>[2x]MKTSKTKTPKSVLIAGPCVIESLENLRSIATKLQPLANNERLDFYFKASFDKANRTSLESYRGPGLEKGLEMLQTIKEEFGYKILTDVHESYQASVAAKVADILQIPAFLCRQTDLIVEVSQTNAIVNIKKGQFMNPKDMQYSVLKALKTRDKSIQSPTYETALKNGVWLCERGS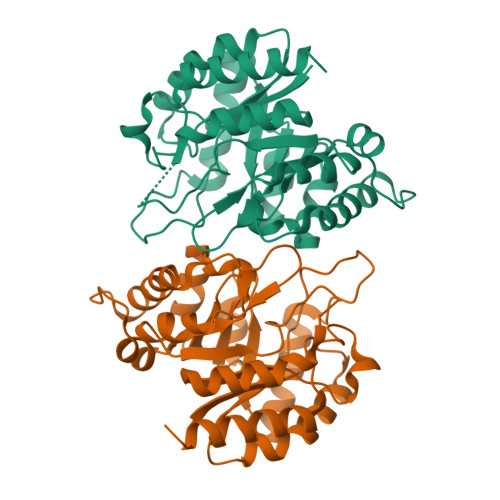SFGYGNLVVDMRSLKIMREFAPVIFDATHSVQMPGGANGKSSGDSSFAPILARAAAAVGIDGLFAETHVDPKNALSDGANMLKPDELEQLVTDMLKIQNLF Human parechovirus 1 is an example of such viruses that contains 60 short regions of ordered RNA density making identical contacts with the protein shell. We show here via a combination of RNA-based systematic evolution of ligands by exponential enrichment, bioinformatics analysis and reverse genetics that these RNA segments are bound to the coat proteins in a sequence-specific manner. Disruption of either the RNA coat protein recognition motif or its contact amino acid residues is deleterious for viral assembly. The data are consistent with RNA packaging signals playing essential roles in virion assembly. Their binding sites on the coat proteins are evolutionarily conserved across the Parechovirus genus, suggesting that they represent potential broad-spectrum anti-viral targets.

The recent HPeV1 X-ray structure at 3.1 Å resolution allows us to answer the question of whether these putative PSs correspond to the ordered RNA segments seen in the virion, and whether they bind to the CP in a sequence-specific fashion. The extent of ordered RNA in the X-ray map is thus significantly less than that in the EM map, but Kalynych et al. could build a model for a 6 nt long RNA (AUUUUU) in the form of an extended single-strand contacting the protein shell. When we examined the deposited electron density map, we found that some of these RNA residues were poorly modelled. The model is an excellent fit and reveals extensive RNA-CP contacts, comprising both hydrogen bond as well as van der Waals contacts. The RNA contacts multiple CP, principally VP3 and VP1. The contacts include three base-specific hydrogen bonds, two to the initial purine, which is therefore confirmed as the consensus G rather than the previously modelled A, although the latter could also be accommodated in this position. There is also a uridine-specific contact to the base N+2 3′ to the G. N+3 is modelled as a uridine which stacks on the side chain of Tyr21, although any base could make this interaction. Amino acid residues in each extended VP3 arm make multiple backbone hydrogen bonds to the RNA fragment neighbouring the one that they contact sequence-specifically, creating a chain of RNA-CP contacts surrounding each five-fold axis. This arrangement strongly suggests that the capsomer for PS binding is a pentamer, because these important recognition sites would not be present on a protomer.

> NSWGSQMDLTDPLCIEDDTENCKQTMSPNELGLTSAQDDGPLGQEKPNYFLNFRSMNVDIFTVSHTKVDNLFGRAWFFMEHTFTNEGQWRVPLEFPKQGHGSLSLLFAYFTGELNIHVLFLSERGFLRVAHTYDTSNDRVNFLSSNGVITVPAGEQMTLSAPYYSNKPLRTVRDNNSLGYLMCKPFLTGTSTGKIEVYLSLRCPNFFFPLPAPKVTSSRALRGDMANLTNQSPY;> APNGKKKNWKKIMTMSTKYKWTRTKIDIAEGPGSMNMANVLCTTGAQSVALVGERAFYDPRTAGSKSRFDDLVKIAQLFSVMADSTTPSENHGVDAKGYFKWSATTAPQSIVHRNIVYLRLFPNLNVFVNSYSYFRGSLVLRLSVYASTFNRGRLRMGFFPNATTDSTSTLDNAIYTICDIGSDNSFEITIPYSFSTWMRKTNGHPIGLFQIEVLNRLTYNSSSPSEVYCIVQGKMGQDARFFCPTGSVVTFQ;> METIKSIADMATGVVSSVDSTINAVNEKVESVGNEIGGNLLTKVADDASNILGPNCFATTAEPENKNVVQATTTVNTTNLTQHPSAPTMPFSPDFSNVDNFHSMAYDITTGDKNPSKLVRLETHEWTPSWARGYQITHVELPKVFWDHQDKPAYGQSRYFAAVRCGFHFQVQVNVNQGTAGSALVVYEPKPVVTYDSKLEFGAFTNLPHVLMNLAETTQADLCIPYVADTNYVKTDSSDLGQLKVYVWTPLSIPTGSANQVDVTILGSLLQLDFQNPRVFAQDVNIYDN The RELATIVE OF EARLY FLOWERING 6 protein (REF6/JMJ12), a Jumonji C (JmjC) domain—containing histone demethylase, specifically demethylates H3K27me3 at its target loci. REF6 has intrinsic DNA-binding ability and specifically recognizes its target sequence (CTCTGYTY motif, Y = T or C) via tandem zinc-finger (ZnF) domains located at its C-terminus. ZnF domains adopt the canonical ββα fold, with a small β-sheet packed against a helix in a globular structure, and wrap more than one turn of the DNA double helix, interacting with DNA in the major groove with a classic α-helix. Structural analysis demonstrates that CHG methylation is unfavorable for REF6 binding and attenuates REF6-binding affinity.

Although the overall structures of the REF6 ZnF domains were similar between complexes with methylated or unmethylated DNA oligos, there are minor conformational changes when DNA strands carrying the methyl-group. Further analysis by isothermal titration calorimetry (ITC) between REF6-ZnFs and the DNA probes with or without 5mCs revealed that 5mCs lead to great reduction in the binding affinity to the CTCTGYTY motif. In combination with EMSA assay, the biochemical and structural studies demonstrated that DNA methylation at the CTCTGYTY-motif, especially at the CTG core, is sufficient to abolish (or severely attenuate) the affinity of REF6-ZnF for this DNA sequence.

>[4x]LMLHKRNICPIKGCGKNFFSHKYLVQHQRVHSDDRPLKCPWKGCKMTFKWAWSRTEHIRVHTGARPYVCAEPDCGQTFRFVSDFSRHKRKTGHSVKKTNKR>[6x]MSHLKNILFIIIVSLFFISSCSTVMSTEGWFMPFDNWLYQLQNADPVEISSSGFEIAVIDYSKDGSESGEYSPEEIKIMVDAGVVPVAYVNIGQAEDYRFYWKESWYTNTPEWLGEEDPAWPGNYFVKYWYNEWKEIVFSYLDRVIDQGFKGIYLDRIDSFEYWAQEGVISRRSAARKMINFVLEIAEYVRERKPDMLIIPQNGENILDFDDGQLASTVSGWAVENLFYLKTIPLEENETKSRLEYLIRLNRKGKFILSVDYVDDGSDSFENISRILDYYEKAKRNGCIPYAARSDLELDEMNVIEGIQPPEALKDYESRTYR

Endo-galactosaminidases are an underexplored family of enzymes involved in the degradation of galactosaminogalactan (GAG) and other galactosamine-containing cationic exopolysaccharides produced by fungi and bacteria. Whereas the fungal enzyme belongs to family GH114, the two bacterial enzymes do not lie in the current GH families but instead define a new family, GH191. The TIM-barrel core structure with fully conserved active-site residues and a negatively charged substrate crevice is conserved among all the families. The putative active-site residues (Asp156/Glu225 for TmGH191, Asp323/Glu391 for Env-GH191 and Asp157/Glu225 for FsGH114) overlap well with the experimentally verified nucleophile and general acid/base Asp189/Glu247 in Ega3, Asp196/Glu222 in Sph3 and Asp160/Glu223 in PelAH.

We could not detect any binding, or enzymatic cleavage of the GAG oligomers, for the T. maritima enzyme, which raises the question as to whether the T. maritima enzyme is an endo-galactosaminidase or whether GAG is not a substrate for this family. The TmGH191 crystals all showed a varying degree of twinning. The structure is composed of tightly packed trimers stacked on each other along their common pseudo-threefold axis. A pair of adjacent trimers form the asymmetric unit, with the two trimers having slightly different orientations (11.5° rotation around the common axis). The stacks of trimers pack into a sparse honeycomb-like structure with wide wells around the pseudo-63 axis and a solvent content of 82.5%. Sph3 has a rather less charged surface due to its activity on neutral GlcNAcylated GAG. A closer inspection shows that the substrate crevice is partially blocked in ‘apo’ TmGH191, especially over the active site via the loop between βi2 and βi3, with Trp121 bridging the active site and blocking access towards the putative −1 subsite. The TmGH191 crystals prepared in this study were soaked with GalN and GalNAc, and a data set was obtained for a GalN-soaked crystal. While no distinct density for a bound carbohydrate was observed, difference density in the substrate-binding crevice of TmGH191 suggests that something has bound, although it could not be conclusively modelled. Some flexibility in the side chain of Trp121 was noted when comparing the native and soaked structures.(7~{R})-7-[(3,5-dimethyl-1,2-oxazol-4-yl)methylamino]-3-[(4-methoxynaphthalen-1-yl)methyl]-5,6,7,8-tetrahydro-[1]benzothiolo[2,3-d]pyrimidin-4-one 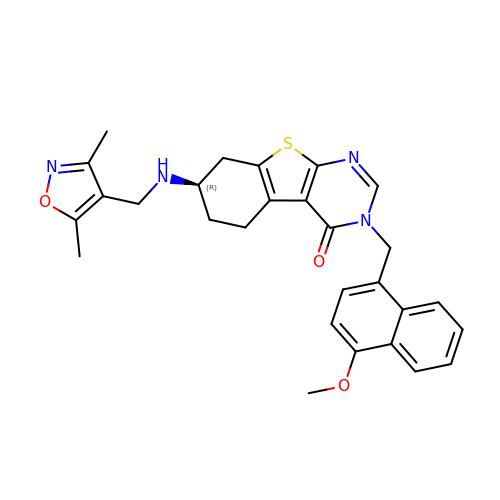| C28 H28 N4 O3 S | HBGRZTNWJBBJHU-LJQANCHMSA-N(4R)-2'-amino-6-(3-chlorophenyl)-1',2,2-trimethyl-2,3-dihydrospiro[chromene-4,4'-imidazol]-5'(1'H)-one | C20 H20 Cl N3 O2 | 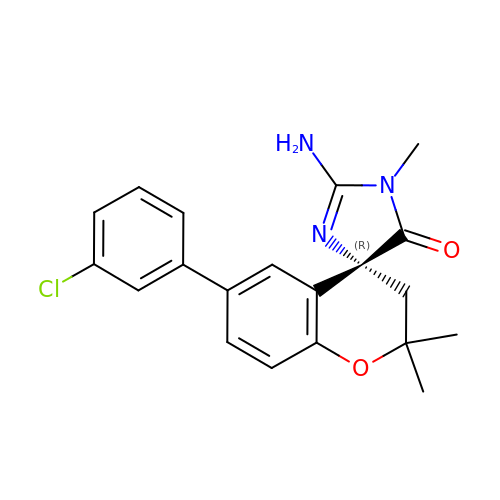MPQDZTDGJUCWQL-HXUWFJFHSA-N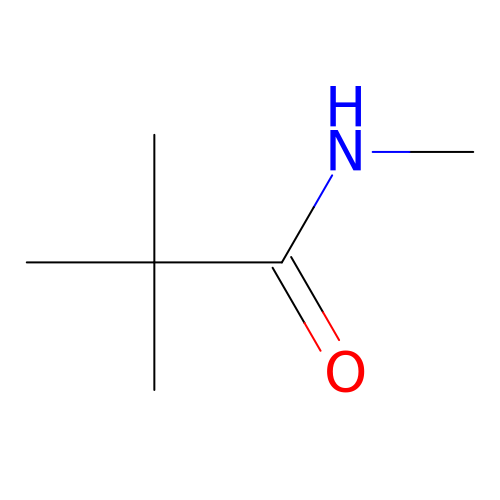N-methyltrimethylacetamide | C6 H13 N O | QMKKJBRRKIKWFK-UHFFFAOYSA-N>MSQLAHNLTLSIFDPVANYRAARIICTIGPSTQSVEALKGLIQSGMSVARMNFSHGSHEYHQTTINNVRQAAAELGVNIAIALDTKGPEIRTGQFVGGDAVMERGATCYVTTDPAFADKGTKDKFYIDYQNLSKVVRPGNYIYIDDGILILQVQSHEDEQTLECTVTNSHTISDRRGVNLPGCDVDLPAVSAKDRVDLQFGVEQGVDMIFASFIRSAEQVGDVRKALGPKGRDIMIICKIENHQGVQNIDSIIEESDGIMVARGDLGVEIPAEKVVVAQKILISKCNVAGKPVICATQMLESMTYNPRPTRAEVSDVANA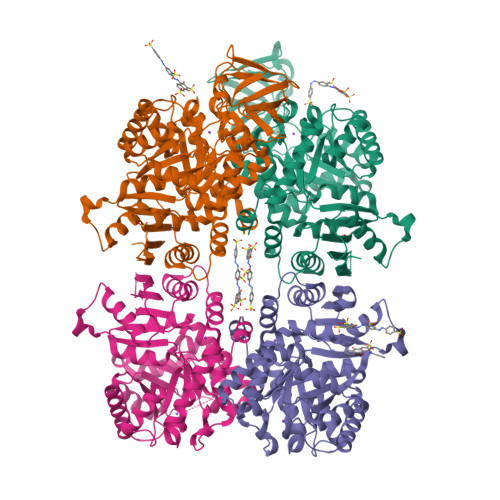VFNGADCVMLSGETAKGKYPNEVVQYMARICLEAQSALNEYVFFNSIKKLQHIPMSADEAVCSSAVNSVYETKAKAMVVLSNTGRSARLVAKYRPNCPIVCVTTRLQTCRQLNITQGVESVFFDADKLGHDEGKEHRVAAGVEFAKSKGYVQTGDYCVVIHADHKVKGYANQTRILLVE[4x]methyl [3-(aminomethyl)-4-(2,4-dichlorophenyl)-2-methyl-7-oxo-5,7-dihydro-6H-pyrrolo[3,4-b]pyridin-6-yl]acetate 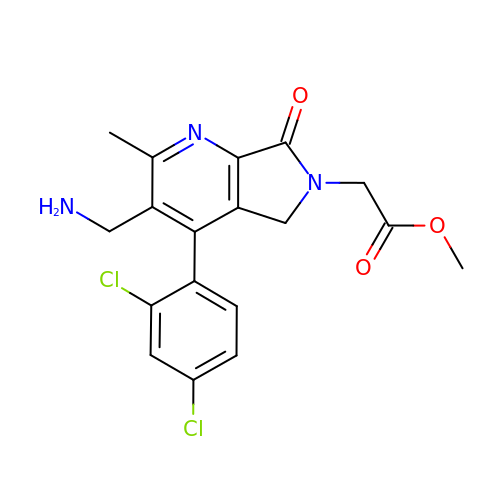| C18 H17 Cl2 N3 O3 | ZPJLWUGRTVIDEI-UHFFFAOYSA-N> MARVAVLISGTGSNLQALIDSTREPNSSAQ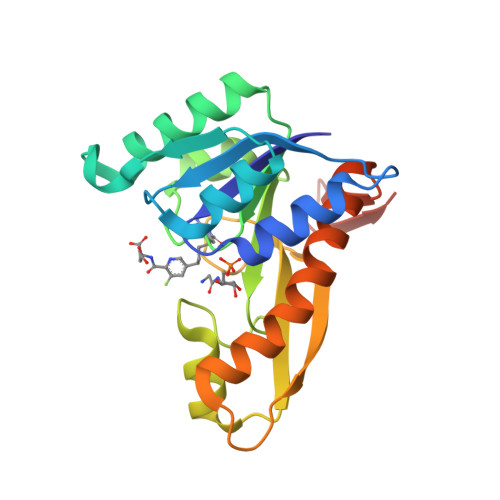IDIVISNKAAVAGLDKAERAGIPTRVINHKLYKNRVEFDSAIDLVLEEFSIDIVCLAGFMRILSGPFVAKWNGKMLNIHPSLLPSFKGSNAHEQALETGVTVTGCTVHFVAEDVDAGQIILQEAVPVKRGDTVATLSERVKLAEHKIFPAALQLVASGTVQLGENGKICWVKEEHHHHHH>[8x]MALDLTAYFDRINYRGATDPTLDVLQDLVTVHSRTIPFENLDPLLGVPVDDLSPQALADKLVLRRRGGYCFEHNGLMGYVLAELGYRVRRF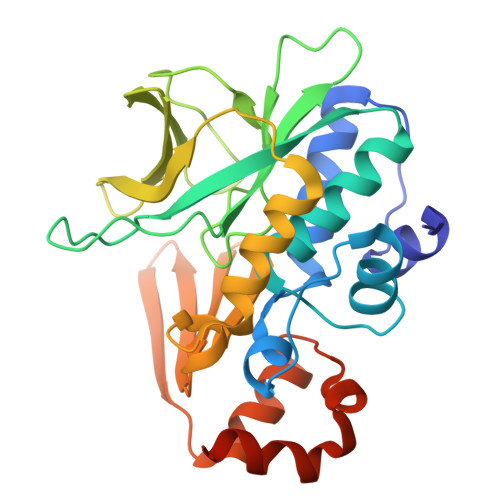AARVVWKLAPDAPLPPQTHTLLGVTFPGSGGCYLVDVGFGGQTPTSPLRLETGAVQPTTHEPYRLEDRVDGFVLQAMVRDTWQTLYEFTTQTRPQIDLKVASWYASTHPASKFVTGLTAAVITDDARWNLSGRDLAVHRAGGTEKIRLADAAAVVDTLSERFGINVADIGERGALETRIDELLARQPGADAP> AVSLDRTRAVFDGSEKSMTLDISNDNKQLPYLAQAWIENENQEKIITGPVIATPPVQRLEPGAKSMVR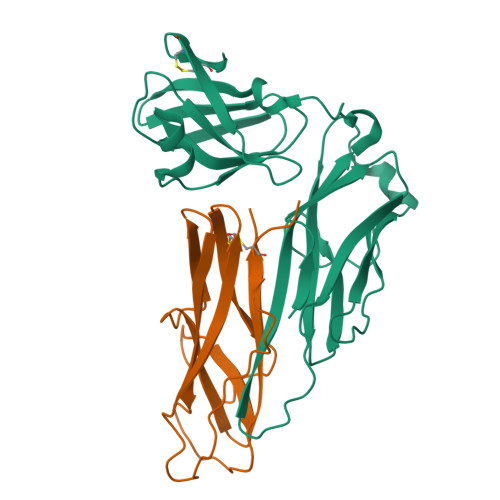LSTTPDISKLPQDRESLFYFNLREIPPRSEKANVLQIALQTKIKLFYRPAAIKTRPNEVWQDQLILNKVSGGYRIENPTPYYVTVIGLGGSEKQAEEGEFETVMLSPRSEQTVKSANYNTPYLSYINDYGGRPVLSFICNGSRCSVKKEKHHHHHH;> IGGCRPSAQSLEIKHGDLSINSANNHYAAQTLSVSCDVPANIRFMLLRNTTPTYSHGKKFSVGLGHGWDSIVSVNGVDTGETTMRWYKAGTQNLTIGSRLYGESSKIQPGVLSGSATLLMILP> MADKRKLQGEIDRCLKKVSEGVEQFEDIWQKLHNAANANQKEKYEADLKKEIKKLQRLRDQIKTWVASNEIKDKRQLIDNRKLIETQMERFKVVERETKTKAYSKEGLGLAQKVDPAQKEKEEVGQWLTNTIDTLNMQVDQFESEVESLSVQTRKKKGDKDKQDRIEGLKRHIEKHRYHVRMLETILRMLDNDSILVDAIRKIKDDVEYYVDSSQDPDFEENEFLYDDLDLEDIPQALVATSPPSHSHMEDEIFNQSSSTPTSTTSSSPIPPSPANCTTENSEDDKKRGRSTDSEVSQSPAKNGSKPVHSNQHPQSPAVPPTYPSGPPPAASALSTTPGNNGVPAPAAPPSALGPKASPAPSHNSGTPAPYAQAVAPPAPSGPSTTQPRPPSVQPSGGGGGGSGGGGSSSSSNSSAGGGAGKQNGATSYSSVVADSPAEVALSSSGGNNASSQALGPPSGPHNPPPSTSKEPSAAAPTGAGGVAPGSGNNSGGPSLLVPLPVNPPSSPTPSFSDAKAAGALLNGPPQFSTAPEIKAPEPLSSLKSMAERAAISSGIEDPVPTLHLTERDIILSSTSAPPASAQPPLQLSEVNIPLSLGVCPLGPVPLPR

Opposing these activities is the CCR4-NOT complex, a highly conserved multi-subunit assembly that functions as the major cytoplasmic deadenylase. mRNA deadenylation rates and half-lives vary by several orders of magnitude and are highly influenced by mechanisms that recruit the CCR4-NOT complex to specific transcripts. The CCR4-NOT complex can also be recruited directly to translating ribosomes to elicit accelerated degradation of specific sets of transcripts. A major trigger for CCR4-NOT recruitment to ribosomes is slow decoding, which is sensed by entry of the N-terminal domain of the CNOT3/Not5 subunit into a vacated E-site when the A-site codon is non-optimal and therefore lacks a cognate tRNA. Here we present our finding that, in mammalian cells, the identity of the P-site tRNA plays a critical role in determining how efficiently CNOT3 is recruited to ribosomes.

Recently, stalling of mammalian ribosomes on a highly non-optimal codon in an in vitro rabbit reticulocyte lysate system was shown to similarly lead to recruitment of CNOT3 to empty E-sites. In the previously reported structures of Not5/CNOT3-bound ribosomes, yeast tRNAiMet or rabbit tRNALeu,UAA, which lack the U13:A22:A46 triplet, occupy the P-site. We therefore examined the Not5/CNOT3-tRNA interaction interfaces in these structures to determine how alternative 13:22:46 triplet configurations affect Not5/CNOT3 binding. tRNAiMet has the most common triplet combination (C13:G22:m7G46), while tRNALeu,UAA has a trans-Hoogsteen G13:A22 pairing characteristic of type-II tRNAs. The distinct base configurations in tRNAiMet and tRNALeu,UAA increase the intermolecular distance to Not5 and CNOT3 in their respective complexes. This prevents the formation of the hydrogen-bonding network observed in our CNOT3/tRNAArg,CCG structure. In our structure, CNOT3 contacts the α element of the D-loop, but not the β element, mirroring the interface between Not5/tRNAiMet in yeast and CNOT3/tRNALeu,UAA in rabbit reticulocyte lysate (and data not shown).>HEHNTIPKGASIEVKVQQLDPVNGNKDVGTVTITESNYGLVFTPDLQGLSAGLHGFHIHENPSCEPKEKEGKLTAGLGAGGHWDPKGAKQHGYPWQDDAHLGDLPALTVLHDGTATNPVLAPRLKHLDDVRGH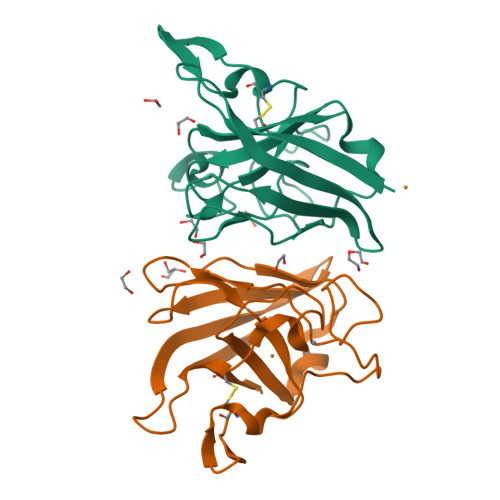SIMIHTGGDNHSDHPAPLGGGGPRMACGVIK[2x]>[2x]KTRIIEFCEFSEEERRRYDDFASKQSVNSLLDENVMKTNLDTNANLAKKKSTAGFVLVQLRKLADHPMLFRIHYKDDILRQMAKAIMNEPQYKKANELYIFEDMQYMSDIELHNLCCKFPSINSFQLKDEPWMDATKVRKLKKLLTNAVENGDRVV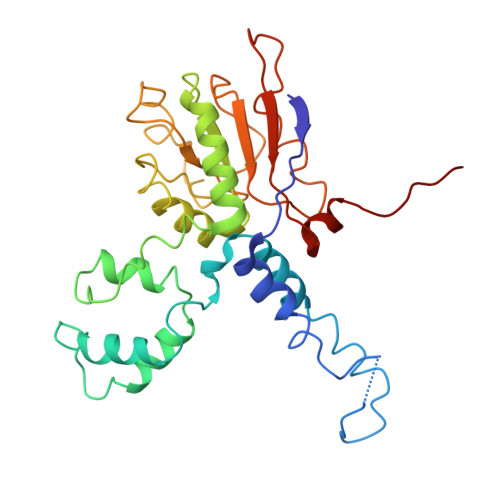LFSQFTQVLDILQLVMKSLNLKFLRFDGSTQVDFRQDLIDQFYADESINVFLLSTKAGGFGINLACANMVILYDVSFNPFDDLQAEDRAHRVGQKKEVTVYKFVVKDTIEEHIQRLANAKIA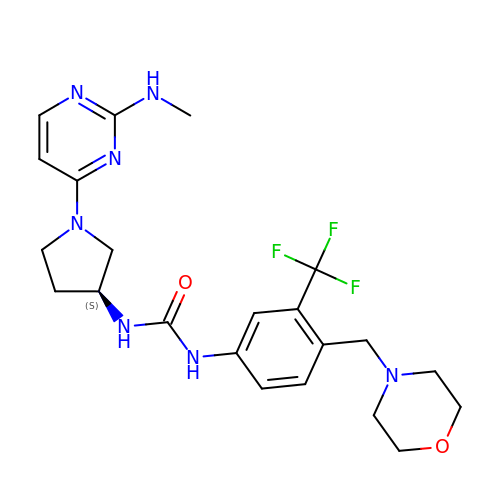N-{(3S)-1-[2-(methylamino)pyrimidin-4-yl]pyrrolidin-3-yl}-N'-{4-[(morpholin-4-yl)methyl]-3-(trifluoromethyl)phenyl}urea | C22 H28 F3 N7 O2 | LVIYMOOJJGCMCP-KRWDZBQOSA-N> LLKALKKL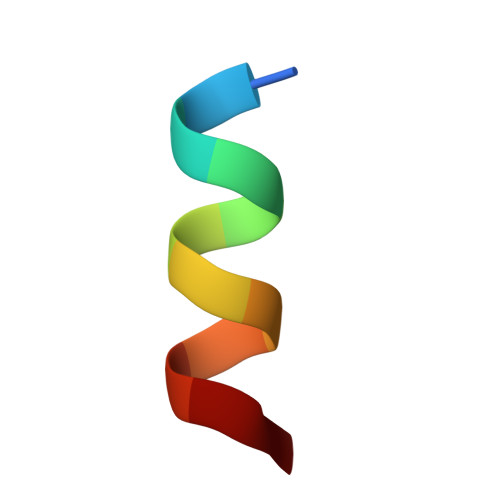AKKY>[2x]YFQSAQTAITDEMLANPPAGEWISYGQNQENYRHSPLTQITTENVGQLQLVWARGMQPGKVQVTPLIHDGVMYLANPGDVIQAIDAKTGDLIWEHRRQLPNIATLNSFGEPTRGMALYGTNVYFVSWDNHLVALDMGTGQVVFDVDRGQGDERVSNSSGPIVANGTIVAGSTCQYSPFGCFVSGHDSATGEELWRNYFIPRAGEEGDETWGNDYESRWMTGAWGQITYDPVTNLVHYGSTAVGPASETQRGTPGGTLYGTNTRFAVRPDTGEIVWRHQTLPRDNWDQECTFEMMVTNVDVQPSTEMEGLQSINPNAATGERRVLTGVPCKTGTMWQFDAETGEFLWARDTNYQNMIESIDENGIVTVNEDAILKELDVEYDVCPTFLGGRDWPSAALNPDSGIYFIPLNNVCYDMMAVDQEFTSMDVYNTSNVTKLPPGKDMIGRIDAIDISTGRTLWSVERAAANYSPVLSTGGGVLFNGGTDRYFRALSQETG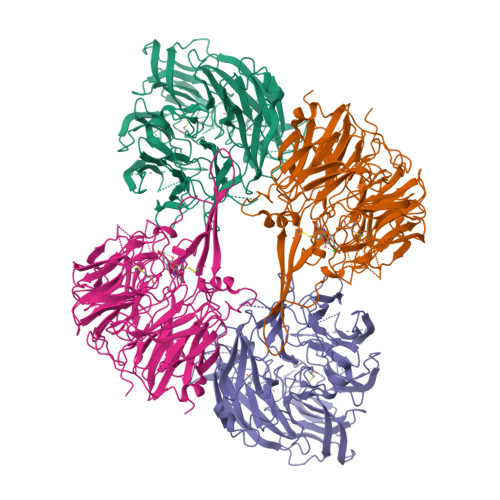ETLWQTRLATVASGQAISYEVDGMQYVAIAGGGVSYGSGLNSALAGERVDSTAIGNAVYVFALPQ>[2x]GSHMSDLPLRFPYGRPEFLGLSQDEVEASADHIARPILILKETRRLPWATG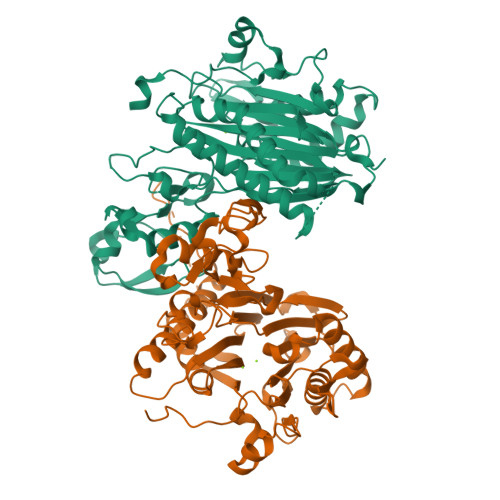YAEVINAGKSTHNEDQASCEVLTVKKKAGAVTSTPNRNSSKRRSSLPNGEGLQLKENSESEGVSCHYWSLFDGHAGSGAAVVASRLLQHHITEQLQDIVDILKNSAVLGSGSTRFFTEKKIPHECLVIGALESAFKEMDLQIERERSSYNISGGCTALIVICLLGKLYVANAGASRAIIIRNGEIIPMSSEFTPETERQRLQYLAFMQPHLLGNEFTHLEFPRRVQRKELGKKMLYRDFNMTGWAYKTIEDEDLKFPLIYGEGKKARVMATIGVTRGLGDHDLKVHDSNIYIKPFLSSAPEVRIYDLSKYDHGSDDVLILATDGLWDVLSNEEVAEAITQFLPNCDPDDPHRYTLAAQDLVMRARGVLKDRGWRISNDRLGSGDDISVYVIPLIHGNKLS>[2x]GPGMATEEMKKLATVMAIGTANPPNCYYQADFPDFYFRVTNSDHLINLKQKFKRLCENSRIEKRYLHVTEEILKENPNIAAYEATSLNVRHKMQVKGVAELGKEAALKAIKEWGQPKSKITHLIVCCLAGVDMPGADYQLTKLLDLDPSVKRFMFYHLGCYAGGTVLRLAKDIAENNKGARVL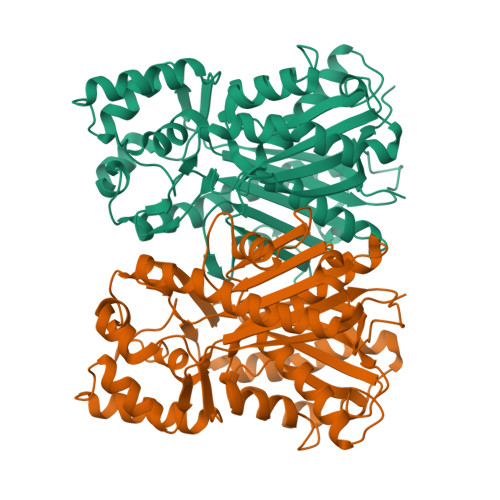IVCSEMTTTCFRGPSETHLDSMIGQALFGDGAAAVIVGADPDLTVERPIFELVSTAQTIVPESHGAIEGHLLESGLSFHLYKTVPTLISNNIKTCLSDAFTPLNISDWNSLFWIAHPGGPAILDQVTAKVGLEKEKLKVTRQVLKDYGNMSSATVFFIMDEMRKKSLENGQATTGEGLEWGVLFGFGPGITVETVVLRSVPVIS> GSAKDPKATTATEHDAFKITTNAKAVPGNYVVEVNKLAQAQTLTTQAKVSDQGAKLGAEGVTDRSLTITAGNPPKETKIPLSDDQ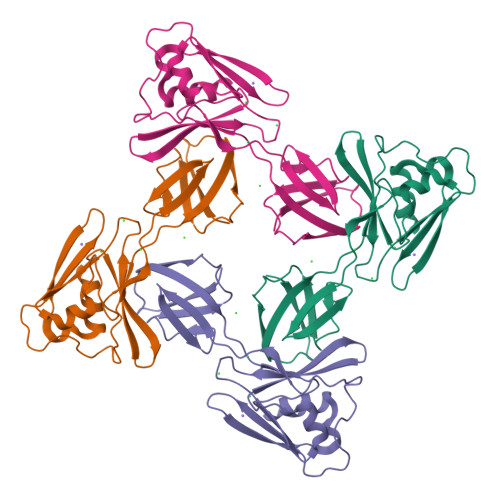TSLVELRDAINGAKAGVTASIMRVGDNDYQLAVSSSTTGENNKISLQVDNDDQLGDILNYNATRGTGTAMKQTVAPQDAELTVNGTAIKRSTNSISDALQGVTIDLKTKTKTDEPQHLVISTN(1S,6R)-10-(1,3-benzothiazol-6-ylsulfonyl)-3-[2-(3,4-dimethoxyphenoxy)ethyl]-3,10-diazabicyclo[4.3.1]decan-2-one 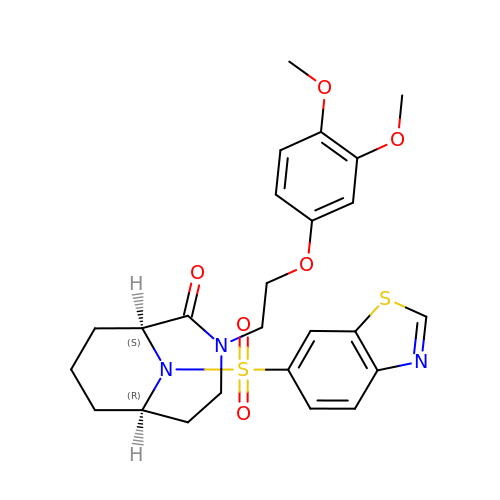| C25 H29 N3 O6 S2 | TYHBYWWSKXMBHC-UTKZUKDTSA-N>[2x]MDPDELPLDEHCERLPYDASKWEFPRDRLKLGKPLGRGAFGQVIEADAFGIDKTATCRTV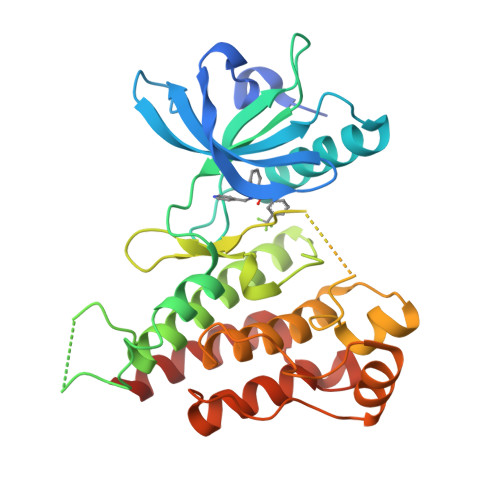AVKMLKEGATHSEHRALMSELKILIHIGHHLNVVNLLGACTKPGGPLMVIVEFCKFGNLSTYLRSKRNEFVPYKVAPEDLYKDFLTLEHLICYSFQVAKGMEFLASRKCIHRDLAARNILLSEKNVVKICDFGLARDIYKDPDYVRKGDARLPLKWMAPETIFDRVYTIQSDVWSFGVLLWEIFSLGASPYPGVKIDEEFCRRLKEGTRMRAPDYTTPEMYQTMLDCWHGEPSQRPTFSELVEHLGNLLQANAQQD>MASNLVEMFNAALNWVTMILESPSARVVLFGVPIRGHFFVEGLLGVVIIILLTRKSYKPPKRPLTEQEIDELCDEWVPEPLIPPITEDMKHEPPVLESAAGPHTTVNGKDVVNFASANYLGLIGHEKLLESCTSALEKYGVGSCGPRGFYGTIDVHLDCETRISKFLGTPDSILYSYGLSTMFSTIPCFCKKGDVIVADEGVHWGIQNGLQLSRSTIVYFKHNDMESLRITLEKIMTKYKRSKNLRRYIVAEAVYQNSGQIAPLDEIVKLKEKYRFRVILDESNSFGVLGRSGRGLAEHHSVPIEKIDVVTAAMGHALATEGGFCTGNARIIDYQRLSSSGYVFSASLPPYLASAAITAIDVIDQNPDMLVKLKQNVALLWKGLSDIKGMSLTSNRESPIVFLKLEKSSGSAKDDLLLLEKMADRALKEDSLLVVSSKRSFLDKCRLPVGIKLYVSAGHSESDLLKASESLKRLASELLLKS[2x];>MITIPYLTAVSTYFSYGLLFAFGQLRDFFRRFIDWWFTSNLQGYAPICLGHEDFYIRRLYHRIQDCFERPISSAPDAWFDVVERYSNDNNKTLKRTTKTSRCLNLGSYNYLGFGSFDEYCTPRVIESLKKFSASTCSSRVDAGTTSVHAELEECVTRFVGKPAAVVFGMGYATNSAIIPVLIGKGGLIISDSLNHSSIVNGARGSGATIRVFQHNTPSHLERVLREQIAEGQPRTHRPWKKIIVVVEGIYSMEGEICHLPEVVAICKKYKAYVYLDEAHSIGAIGKTGKGICELLGVDTADVDVMMGTFTKSFGSCGGYIAGSKELIQYLKHQCPAHLYATSIPTPSAQQIISAIKVILGEDGSNRGAQKLARIRENSNFFRAELQKMGFEVLGDNDSPVMPIMLYNPAKIPAFSRECLRQKVAVVVVGFPATPLLLARARICISASHSREDLIRALKVISKVGDLSGIKYFPAEPKKIEQSKNDIKLD[2x];>[2x]MADYKDDDDKSGPDEVDASGRMNWVQRKIYLYNVTFGLYMLDWWERYLFNSLVVVLMWFVLYNGTRYFSELFQRHLT;>MANLYVKAVPPPDMNRNTEWFMYPGVWTTYMLILFFGWLVVLSVSGCSPGMAWTVVNLAHFVVTYHSFHWMKGTPFADDQGIYNGLTWWEQMDNGQQLTRNRKFLTLVPVVLYLIASHTTDYRHP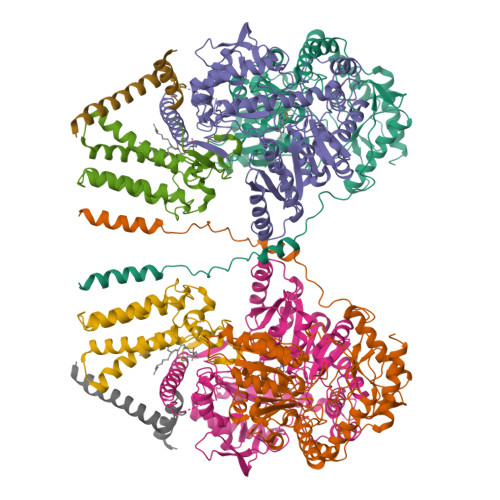WLFLNTLAVMVLVVAKFPNMHKVRIFGINGDK[2x]R-STYRENE OXIDE | C8 H8 O | 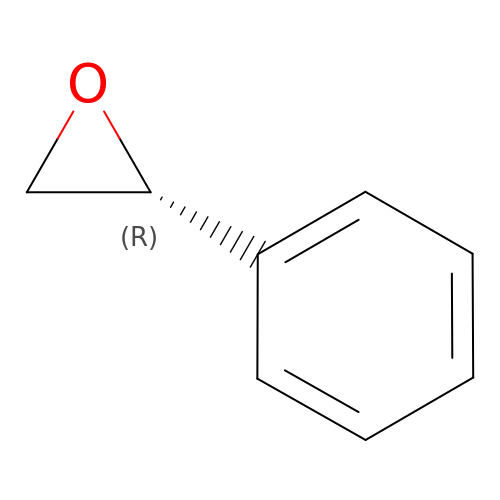AWMVMTVKBNGEAK-QMMMGPOBSA-N>MSKLIVPQWPQPKGVAACSSTRIGGVSLPPYDSLNLGAHCGDNPDHVEENRKRLFAAGNLPSKPVWLEQVHGKDVLKLTGEPYASKRADASYSNTPGTVCAVMTADALPVLFCNRAGTEVAAAHAGWRGLCAGVLEETVSCFADNPENILAWLGPAIGPRAFEVGGEVREAFMAVDAKASAAFIQHGDKYLADIYQLARQRLANVGVEQIFGGDRCTYTENETFFSYRRDKTTGRMASFIWLILEHHHHHH[4x]

YfiH is a PG-editing factor whose absence causes misincorporation of l-Ser instead of l-Ala into peptide stems, but its mechanistic function is unknown. Here, we report the crystal structures of substrate-bound and product-bound YfiH, showing that YfiH is a cytoplasmic amidase that controls the incorporation of the correct amino acid to the nucleotide precursors by preferentially cleaving the nucleotide precursor by-product UDP–MurNAc–l-Ser. Our results show that YfiH forms an extended L-shaped binding groove for the UDP-MurNAc-monopeptide and is a cytoplasmic amidase specific for hydrolyzing UDP–MurNAc–l-Ser, a noncanonical reaction by-product from the MurC reaction. Our results showing YfiH as an l-Ser-specific UDP-MurNAc-monopeptide amidase therefore uncover a bacterial control mechanism to ensure only the presence of the specific amino acid in the peptide assembly pathways by removing unwanted UDP-MurNAc-monopeptide byproducts from the MurC reactions.

We expressed catalytically inactive recombinant E. coli YfiH-C107A protein for the original purpose of screening potential substrates or ligands by binding assays and cocrystallography. Purified YfiH-C107A forms highly diffracting crystals; the best crystal diffracted to a 1.47-Å resolution in the space group P212121, with four molecules (chains A to D) per asymmetric unit. Serendipitously, the electron density map contained a prominent blob of well-resolved density for an endogenous compound, presumably copurified with YfiH-C107A and trapped during crystallogenesis. This compound was unambiguously identified as UDP-MurNAc based on its high-resolution map. The structure of UDP-MurNAc-bound E. coli YfiH adopts an overall globular structure that features a pair of two central β-sheets sandwiched by multiple α-helices, which is similar to the structures of Shigella flexneri YfiH and Geobacillus stearothermophilus YlmD (with root mean square difference [RMSD] values of 0.9 Å and 1.3 Å, respectively). UDP-MurNAc is bound to a preformed groove located on one side of the double β-sheets and at a distinct β-turn (aa 104 to 108). The β-turn bridges the two β-sheets; importantly, it harbors the catalytic Cys107 and forms the oxyanion hole by the backbone amides of Ala105 and Asp106. UDP-MurNAc forms a largely extended conformation in the elongated L-shaped binding groove of YfiH, where the uridine moiety forms a sharp angle with the diphosphate-linked MurNAc. The aromatic ring of uracil packs against the side chain of Arg228 from H7, forming the turning point of the groove. The lactyl oxygens of MurNAc interact with His71 from L3 and His124, which forms a catalytic triad with Asp89 and Cys107.> GDDLEVGKNIDESAYSGIYENNAYLRDGKSNLVSKVVELHGETYATTVKMGLSKTPNTATSAKVKIDAAYLETYNKAHNTDFALYPQDLVTFANEGILTVNANTKSAEVEMTIRAGEGLQEDKTYAIPVAISDQSSDITIKDEDAKHCIYLVKDMRNAGDAYKGEGVMQGYLFFEVNDVNPLNTLSFQLENGKLLWDVVVLFAANINYDAEAGRPRVQCNPNVQYLLDNNETLLQPLRRRGVKVLLGLLGNHDITGLAQLSEQGAKDFAREVAQYCKAYNLDGVNYDDEYSNSPDLSNPSLTNPSTAAAARLCYETKQAMPDKLVTVFDWGQMYGVATVDGVDAKEWIDIVVANYGSAAYPIGQMTKKQCSGISMEFNLGGGGSLSASKAQSMIDGGYGWFMGFAPSPAKYGSVFSRLQGGGEVLYGSNVAAPTIFYKKNDPTPYKYPDDL

ENGases are endoglycosidases that hydrolyze the β(1,4) linkage between the first two GlcNAc residues of N-linked glycans on proteins. To this end, we focus on two GH18 enzymes, EndoS2 from S. pyogenes and EndoBT-3987 from Bacteroides thetaiotaomicron, a key enzyme that catalyzes the first step in the degradation and processing of mammalian HM-type N-glycans in the human gut. EndoBT-3987 is composed of two domains: the N-terminal β-sandwich domain (residues 42–179) and the C-terminal glycoside hydrolase domain, which adopts an (α/β)8-barrel topology typical of GH18 family enzymes (residues 194–476). D312 stabilizes the reaction intermediate by hydrogen bond interaction and orients the oxygen of the 2-acetamide group of GlcNAc (−1) in order to attack the anomeric carbon, forming the oxazoline intermediate, whereas E314 acts as an acid/base, protonating the anomeric carbon in this first step and in a second step deprotonating a water molecule that produces the second nucleophilic attack.

Here we present the X-ray crystal structure of the ENGase EndoBT-3987 from Bacteroides thetaiotaomicron in complex with a hybrid-type glycan product. We unambiguously identified the Hy-type N-glycan product in the electron density map, located at the center of the glycoside hydrolase domain in a shallow pocket decorated by the connecting loops β10–α2 (loop 1; residues 201–205), β11–α3 (loop 2; residues 228–245), β14–α4 (loop 3; residues 275–286), β15–α5 (loop 4; residues 313–330), β16–β17 (loop 5; residues 355–374), β17–β18 (loop 6; residues 379–395), β18–α6 (loop 7; residues 402–411), and β19–α7 (loop 8; residues 430–432). We could not reliably model the terminal Neu5Ac (−9), suggesting that this residue is solvent exposed and adopts multiple conformations in the crystal. In the EndoBT-3987WT-Hy product crystal structure, all the sugar residues are in the energetically favorable chair conformation 4C1 but GlcNAc (−1) residue is in skew boat conformation (1S3) stabilized by interactions with protein residues. The nitrogen and oxygen atoms of the acetamide group of GlcNAc (−1) make hydrogen bonds with the side chains of Y380 and D312, respectively. The base of the binding site is mainly composed of a set of aromatic hydrophobic residues, including F198, F227, F353, and F429, located at the top of the corresponding β10, β11, β16, and β19 β-strands of the barrel, respectively. The α(1,6) antenna (Manα1–6(Manα1–3)Manα1–6) interacts with loops 1, 2, 3, and 4, whereas the α(1,3) antenna (Galβ1–4GlcNAcβ1–2Manα1–3) is largely solvent exposed and interacts with loops 1 and 7 of EndoBT-3987, mainly through Man (−6) and GlcNAc (−7) residues. Man (−5) is completely buried into the binding site. The O2 and O6 atoms of Man (−5) make hydrogen bonds with the side chains of N202 and E200, respectively. In contrast, the interaction of EndoBT-3987 with Hy-type N-glycans is driven by the α(1,6) antenna.>SMMELRVGNRYRLGRKIGSGSFGDIYLGTDIAAGEEVAIKLECVKTKHPQLHIESKIYKMMQGGVGIPTIRWCGAEGDYNVMVMELLGPSLEDLFNFCSRKFSLKTVLLLADQMISRIEYIHSKNFIHRDVKPDNFLMGLGKKGNLVYIIDFGLAKKYRDARTHQHIPYRENKNLTGTARYASINTHLGIEQSRRDDLESLGYVLMYFNLGSLPWQGLKAATKRQKYERISEKKMSTPIEVLCKGYPSEFATYLNFCRSLRFDDKPDYSYLRQLFRNL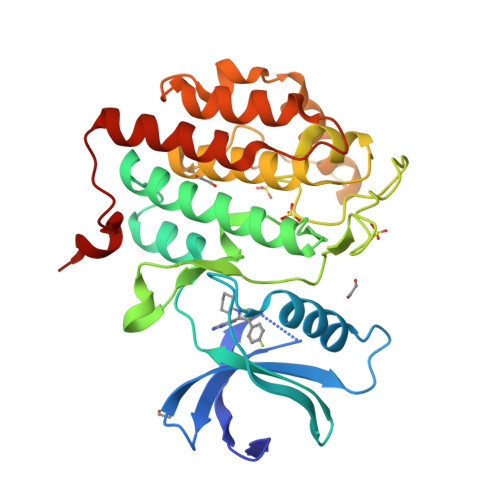FHRQGFSYDYVFDWNMLK[4x]> MDLLAELQWRGLVNQTTDEDGLRKLLNEERVTLYCGFDPTADSLHIGHLAGILTMRRFQQAGHRPIALVGGATGLIGDPSGKKSERTLNAKETVEAWSARIKEQLGRFLDFEADGNPAKIKNNYDWIGPLDVITFLRDVGKHFSVNYMMAKESVQSRIETGISFTEFSYMMLQAYDFLRLYETEGCRLQIGGSDQWGNITAGLELIRKTKGEARAFGLTIPLVTKADGTKFGKTESGTI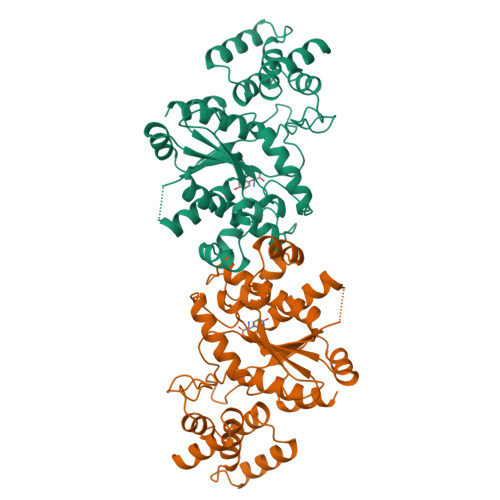WLDKEKTSPYEFYQFWINTDDRDVIRYLKYFTFLSKEEIEALEQELREAPEKRAAQKTLAEEVTKLVHGEEALRQAIRIS>[2x]MASTNKDQITLSSSPIFISTENLRTILTHQTLINHIQSNLPKASTFLQTPIRQHYNLSPSSSLLLMPSW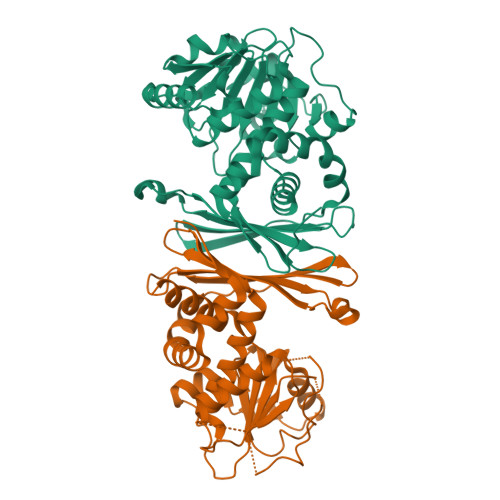SSTPSFPYIGVKLVTHFPENSSQNLPGVQGSYVLFNSTTGQTLASMDSTELTLYRTSCVSGLASKYLARDDSEILVMVGAGALAPHLIKAHFSARPSLKKVFIWNRTVEKAINLAKKLSESDEFPLSGLSFEGCGNLDEVVGFGDIVSCATNSEAALVKGERLKVGAHLDLVGSFKHSMKECDDEALKRGKVFVDNEAALVEAGELVGAFERGVIKEDEIGGNLLELIRGDKVGRSSSEEITVFKSVGSAVVDMLAAQFVYETYTRT> MIGRLLRGGFMTAIYAYLYIPIIILIVNSFNSSRFGINWQGFTTKWYSLLMNNDSLLQAAQHSLTMAVFSATFATLIGSLTAVALYRYRFRGKPFVSGMLFVVMMSPDIVMAISLLVLFMLLGIQLGFWSLLFSHITFCLPFVVVTVYSRLKGFDVRMLEAAKDLG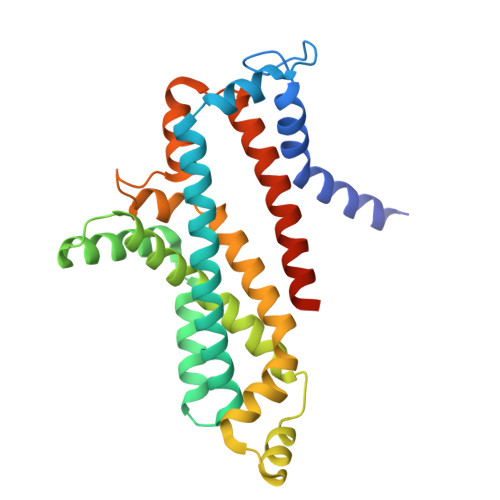ASEFTILRKIILPLAMPAVAAGWVLSFTLSMDDVVVSSFVTGPSYEILPLKIYSMVKVGVSPEVNALATILLVLSLVMVIASQLIARDKTKGNTGDVK4-[3-(phenylsulfonylamino)prop-1-ynyl]-~{N}-[3,3,3-tris(fluoranyl)propyl]benzenesulfonamide 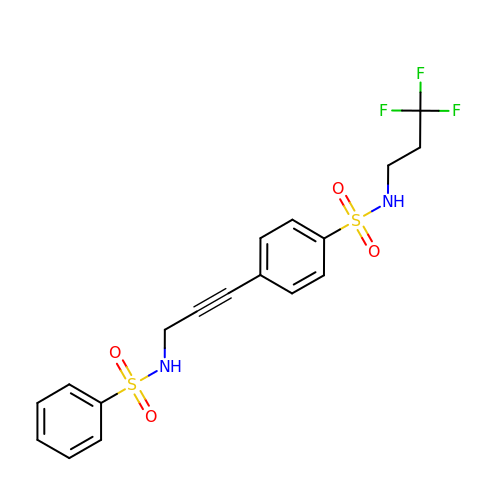| C18 H17 F3 N2 O4 S2 | YOHZJJJIFGXOPP-UHFFFAOYSA-N>GPGSMAGVDKAMVTLSNGVKMPQFGLGVWQSPAG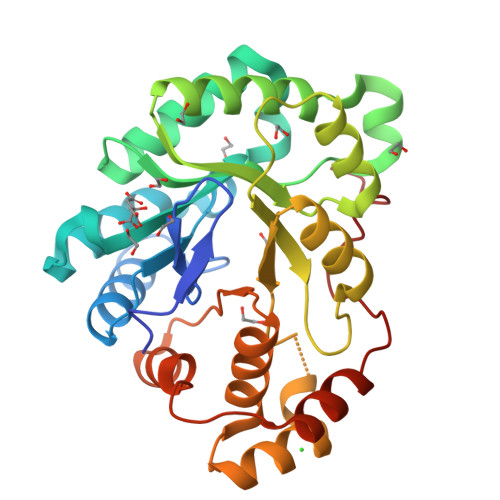EVTENAVKWALCAGYRHIDTAAIYKNEESVGAGLRASGVPREDVFITTKLWNTEQGYESTLAAFEESRQKLGVDYIDLYLIHWPRGKDILSKEGKKYLDSWRAFEQLYKEKKVRAIGVSNFHIHHLEDVLAMCTVTPMVNQVELHPLNNQADLRAFCDAKQIKVEAWSPLGQGKLLSNPILSAIGAKYNKTAAQVILRWNIQKNLITIPKSVHRERIEENADIFDFELGAEDVMSIDALNTNSRYGPDPDEAQF[2x]5'-O-[(R)-hydroxy{[2-hydroxy-3,5-dimethyl-6-(2-oxo-2-sulfanylethyl)pyridin-4-yl]oxy}phosphoryl]guanosine | C19 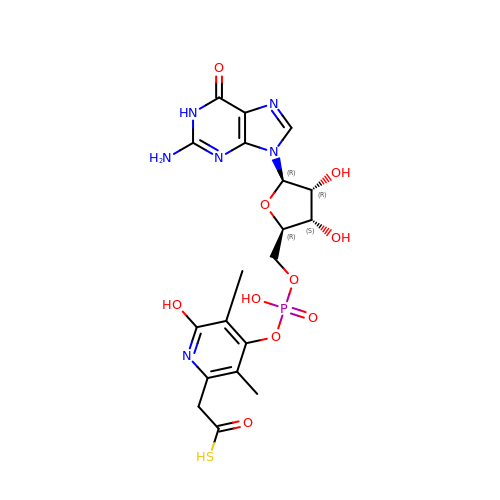H23 N6 O10 P S | JZNXQNYXQOKUIF-ACDAHVMNSA-N>[2x]MGSHHHHHHSSGLVPRGSHSDEVDAHMMQLHKPDVVAAATKILDDHGIADLTMRRLARELDVTPGALYWHFANKQELLGAVA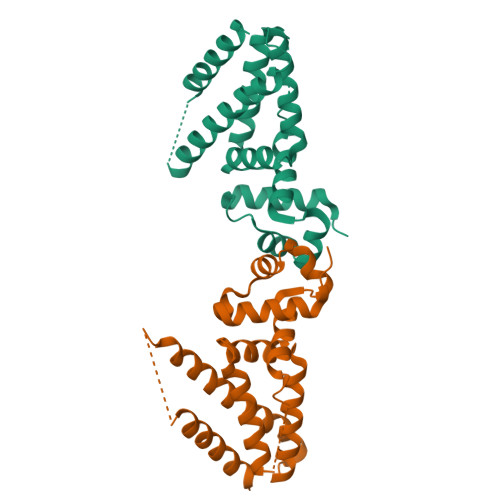DHILRTARTDTADLAWREQIHESCRALRDALLSHTDGAELVSASFASGQSVVITEIVEQLGRAARAAGVSDADVDAAARTVIYYVLGFTVDEQSRLQWDAVGALGDDQSMLTRDGTRQFRFGLQLLVDGLAAHGGGSEFTGFSSAERSFE>GMLEARLEQASLLKRVVDAIKDLVQDCNFDCNDSGIALQAMDNSHVA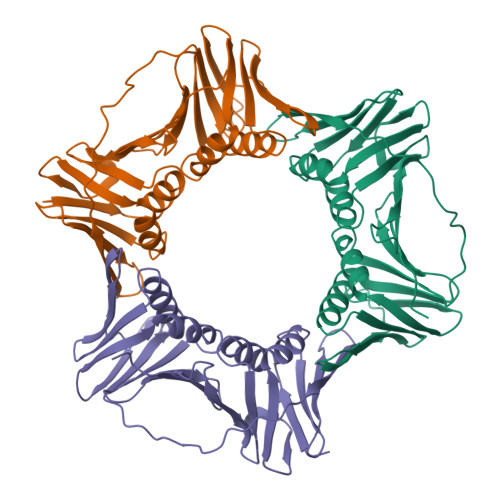LVSMLLKAEGFSPYRCDRNIALGINLVSLTKVLRAAQNEDILTLKADDSPDAVNLMFESAETDRISEYDIKLMDIDQEHLAIPETEYAATVEMPSAEFQRICRDLNALSESVVIEATKEGVKFSCQGDIGSGSVTIRQHTSVDKPEQNVSIALSEPVALTFSLKYLVNFCKATSLSSKVTLCLSQEVPLLVEYGLGSGHLRFYLAPKIGDEE[3x]>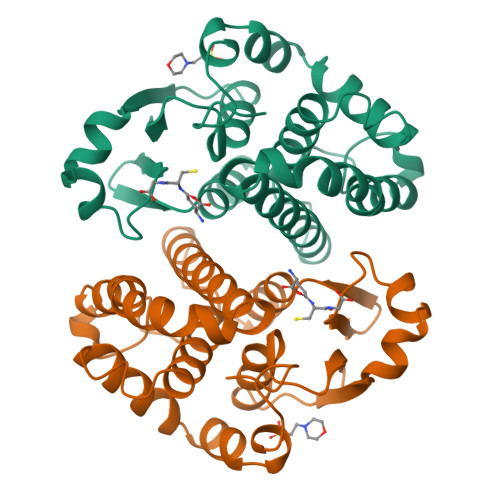PPYTVVYFPVRGRCAALRMLLADQGQSWKEEVVTVETWQEGSLKASCLYGQLPKFQDGDLTLYQSNTILRHLGRTLGLYGKDQQEAALVDMVNDGVEDLRCKYISLIYTNYEAGKDDYVKALPGQLKPFETLLSQNQGGKTFIVGDQISFADYNLLDLLLIHEVLAPGCLDAFPLLSAYVGRLSARPKLKAFLASPEYVNLPINGNGKQ[4x]> GTFTWTLSDSEGKDTPGGYCLTRWMLIEAELKCFGNTAVAKCNEKHDEEFCDMLRLFDFNKQAIQRLKAEAQMSIQLINKAVNALINDQLIMKNHLRDIMGIPYCNYSKYWYLNHTTTGRTSLPKCWLVSNGSYLNETHFSDDIEQQADNMITEMLQKEYMERQGKT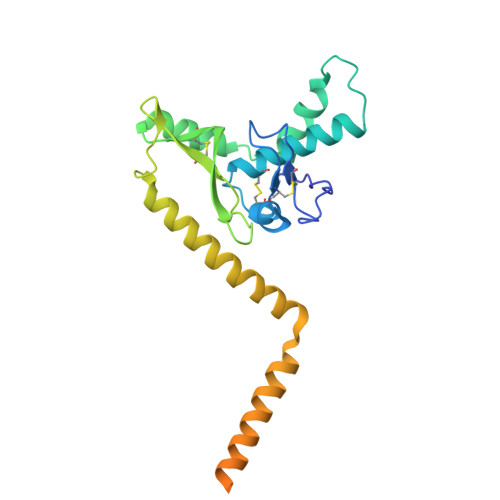PLGLVDLFVFSTSFYLISIFLHLVKIPTHRHIVGKSCPKPHRLNHMGICSCGLYKQPGVPVKWKRGGGSDYKDDDDK>MSDQLQMTDGMHIIVEALKQNNIDTIYGVVGIPVTDMARHAQAEGIRYIGFRHEQSAGYAAAASGFLTQKPGICLTVSAPGFLNGLTALANATVNGFPMIMISGSSDRAIVDLQQGDYEELDQMN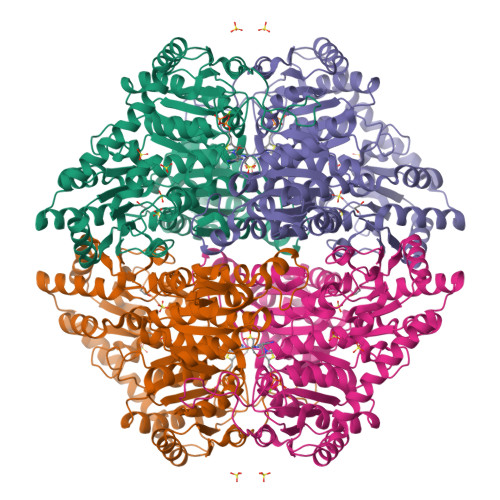AAKPYAKAAFRVNQPQDLGIALARAIRVSVSGRPGGVYLDLPANVLAATMEKDEALTTIVKVENPSPALLPCPKSVTSAISLLAKAERPLIILGKGAAYSQADEQLREFIESAQIPFLPMSMAKGILEDTHPLSAAAARSFALANADVVMLVGARLNWLLAHGKKGWAADTQFIQLDIEPQEIDSNRPIAVPVVGDIASSMQGMLAELKQNTFTTPLVWRDILNIHKQQNAQKMHEKLSTDTQPLNYFNALSAVRDVLRENQDIYLVNEGANTLDNARNIIDMYKPRRRLDCGTWGVMGIGMGYAIGASVTSGSPVVAIEGDSAFGFSGMEIETICRYNLPVTIVIFNNGGIYRGDGVDLSGAGAPSPTDLLHHARYDKLMDAFRGVGYNVTTTDELRHALTTGIQSRKPTIINVVIDPAAGTESGHITKLNPKQVAGN[2x]> MSELLDSFETEFAKFYTDSNLEETNLQKCLDHTHEFKSQLKKLKAHLNKHIQESKPEVYNKLSDKEKQKFKRKRELIIEKLSKSQRQWDHSVKKQIKYV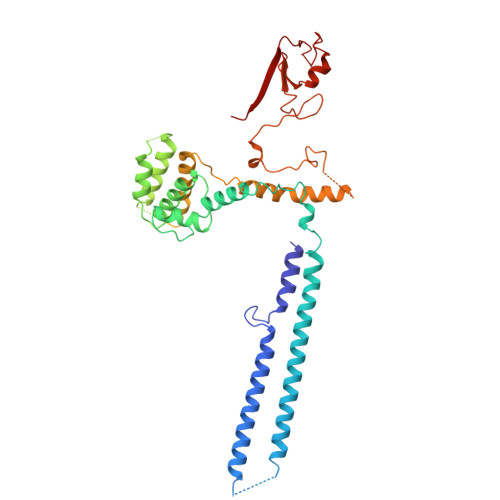SQQSNRFNKSTLNKLKEFDIDSVYVNKLPKETMENVNEAIGYHILRYSIDNMPLGNKNEAFQYLKDVYGITNKESTEFIEMGQIVHDLKKGDTESCLKWCSNEMESLSSNHTALSSLKFDLYTLSAMQIVKHGNPVELYYQITQNAPLDCFRHREKELMQNVVPLLTKSLIGQPIEDIDSKVNKELKECTSLFIKEYCAAKHIFFDSPLFLIVLSGLISFQFFIKYKTIRELAHVDWTTKDELPFDVKLPDFLTHFHPIFICPVLKEETTTENPPYSLACHHIISKKALDRLSKNGTITFKCPYCPVNTSMSSTKKVRFVML>EEKDEEFPEQKAGEAINQPMMMAARQLHDEARKWSSKGNDIIAAAKRMALLMAEMSRLVRGGSGNKRALIQCAKDIAKASDEVTRLAKEVAKQCTDKRIRTNLLQVCERIPTISTQLKILSTVKATMLGRTNISDEESEQATEMLVHNAQNLMQSVKETVREAEAASIKIRTDAGFTLR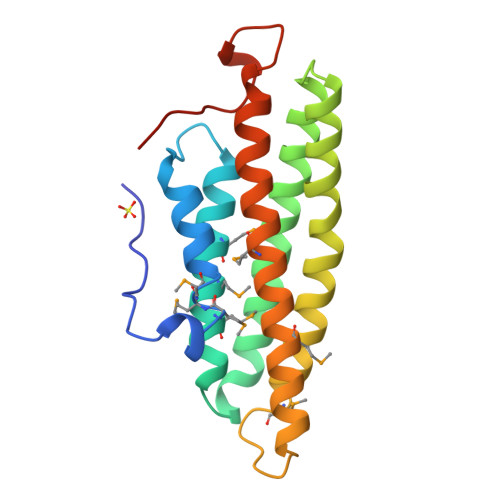WVRKTPWYQ[2x]> MESKRNKPGKATGKGKP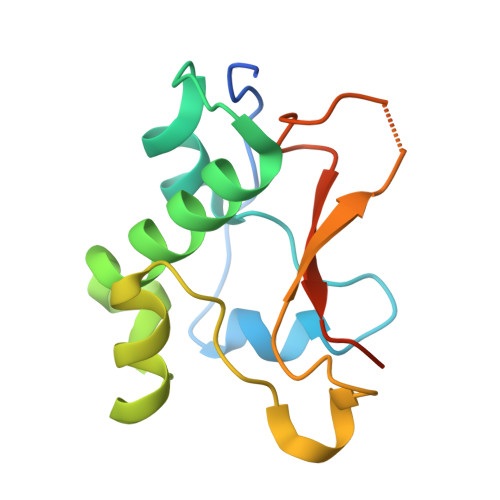VGDKWLDDAGKDSGAPIPDRIADKLRDKEFKSFDDFRKAVWEEVSKDPELSKNLNPSNKSSVSKGYSPFTPKNQQVGCRKVYELHHDKPISQGGEVYDMDNIRVTTPKRHIDIHRGK> NSFVGLRVVAKWSSNGYFYSGKITRDVGAGKYKLLFDDGYECDV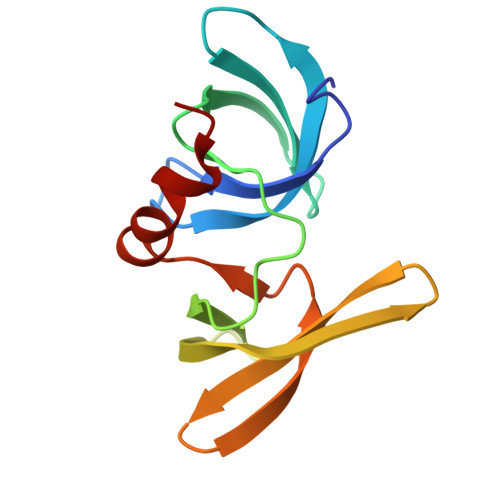LGKDILLCDPIPLDTEVTALSEDEYFSAGVVKGHRKESGELYYSIEKEGQRKWYKRMAVILSLEQGNRLREQYGLG>MDKFRVQGPTKLQGEVTISGAKNAALPILFAALLAEEPVEIQNVPKLKDVDTSMKLLSQLGAKVERDGSVHIDARDVNVFCAPYDLVKTMRASIWALGPLVARFGQGQVSLPGGCTIGARPVDLHISGLEQLGATIKLEEGYVKASVDGRLKGAHIVMDKVSVGATVTIMCAATLAEGTTIIENAAREPEIVDTANFLITLGAKISGQGTDRIVIEGVERLGGGVYRVLPDRIETGTFLVAAAISRGKIICRNAQPDTLDAVLAKLRDAGADIEVGEDWISLDMHGKRPKAVNVRTAPHPAFPTDMQAQFTLLNLVAEGTGFITETVFENRFMHVPELSRMGAHAEIESNTVICHGVEKLSGAQVMATD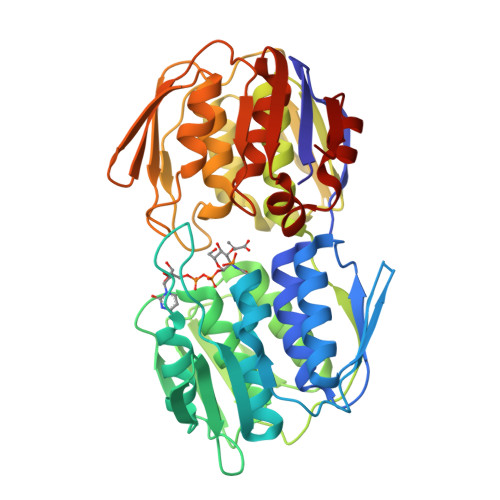LRASASLVLAGCIAEGTTVVDRIYHIDRGYERIEDKLRALGANIERVKG[12x]> MAPSPDPPPVIKMFNRHMLFDIVSRGSTAELEGFLPFLLAQKKRLTDEEFREASTGKTCLTKALMNLNGGKNDTIPMLIDIAEKTGNLREFINSPFRDVYYRGQTALHIAIERRCKHYVELLVEKGADVHAQARGRFFQPKDEGGYFYFGELPLSLAACTNQPDIVHYLTENAHKKADIRRQDSRGNTVLHALVAIADNTRENTKFVTKVYDLLVIKCVKLYPDSSLEAIFNNDSMSPLMMAAKLGKIGIFQHIIRLEIKDEEARHLSRKFRDWAYGPVYSSLYDLSMLDTCGEEVSVLEILVYNSKVENRHEMLAVEPINELLRDKWQKFGAVSFYISVVSYLIAMIIFTLIAYYRPMDGTPPYPYRTTMDYMRLAGEIVTLLTGVVFFITNIKDLFMKKCPGVNSLFIDGSFQLLYFIYSVLVIITAVLYLV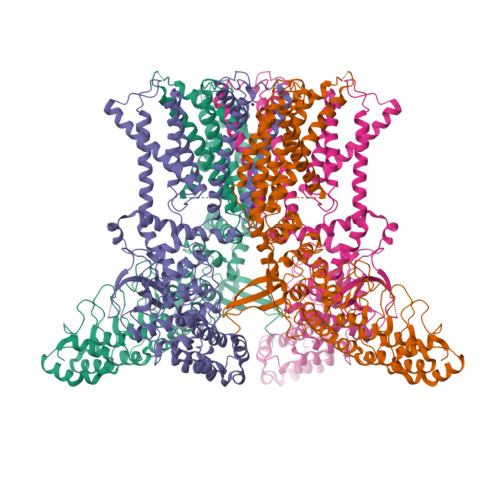GIESYLAVMVFALVLGWMNALYFTRGLKLTGTYSIMLQKILFKDLFRFLLVYLLFMIGYASALVSLLNPCTSQESCIETSSQCTVPEYPSCRDSSTFSKFLLDLFKLTIGMGDLEMINSAKYPAVFIILLVTYIILTFVLLLNMLIALMGETVGQVSKESKQIWKLQWATTILDIERSFPVCMRKAFRSGEMVTVGKNLDGTPDRRWCFRVDEVNWSHWNQNLGIINEDPGRSNSLEVLFQ>GEFTQSVSRLQSIVAGLKNAPSDQLINIFESCVRNPVENIMKILKGIGETF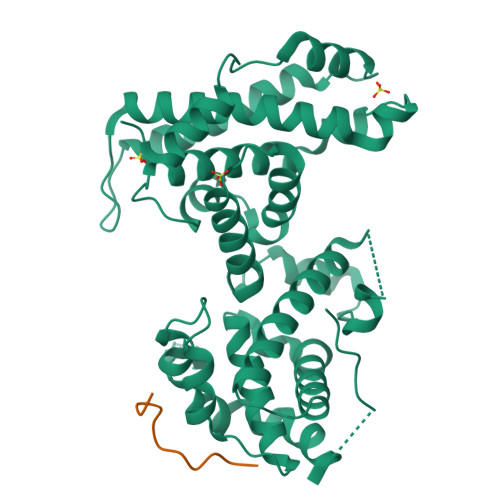CQHYTQSTDEQPGSHIDFAVNRLKLAEILYYKILETVMVQETRRLHGMDMSVLLEQDIFHRSLMACCLEIVLFAYSSPRTFPWIIEVLNLQPFYFYKVIEVVIRSEEGLSRDMVKHLNSIEEQILESLAWSHDSALWEALQVSANKVPTCEEVIFPNNFETGNNRPKRTGSLALFYRKVYHLASVRLRDLCLKLDVSNELRRKIWTCFEFTLVHCPDLMKDRHLDQLLLCAFYIMAKVTKEERTFQEIMKSYRNQPQANSHVYRSVLLKSIKEERGDLIKFYNTIYVGRVKSFALKYDLANQDHMMDAPPLSPFPHIKQQ[2x];>[2x]GPETLVCHEVDLDDL> GHMFQCNVPLGMESGRIANEQISASSTYSDGRWTPQQSRLHGDDNGWTPNLDSNKEYLQVDLRFLTMLTAIATQGAISRETQNGYYV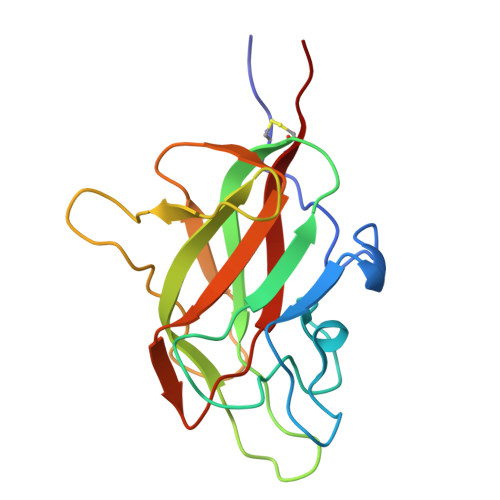KSYKLEVSTNGEDWMVYRHGKNHKVFQANNDATEVVLNKLHAPLLTRFVRIRPQTWHSGIALRLELFGCRVTSGS>[2x]SNHHRGLASANVDFAFSLYKHLVALSPKKNIFISPVSISMALAMLSLGTCGHTRAQLLQGLGFNLTERSETEIHQGFQHLHQLFAKSDTSLEMTMGNALFLDGSLELLESFSADIKHYYESEVLAMNFQDWATASRQINSYVKNKTQGKIVDLFSGLDSPAILVLVNYIFFKGTWTQPFDLASTREENFYVDETTVVKVPMM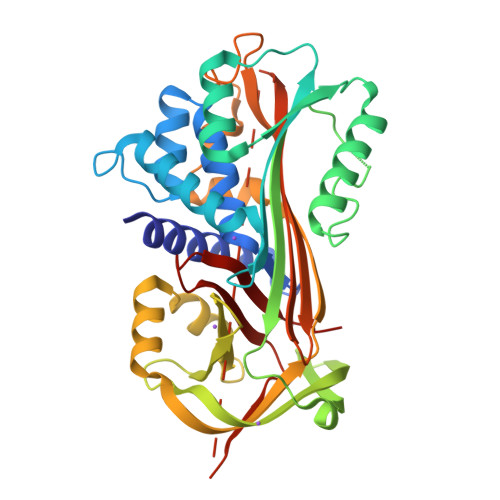LQSSTISYLHDSELPCQLVQMNYVGNGTVFFILPDKGKMNTVIAALSRDTINRWSAGLTSSQVDLYIPKVTISGVYDLGDVLEEMGIADLFTTQANFSRITQDAQLKSSKVVHKAVLQLNEEGTEAAGAMFLEAIPRSKPIILRFNQPFIIMIFDHFTWSSLFLARVMNPV> SHMVVLGGDRDFWLQVGIDPIQIMTGTATFYTLRCYLDDRPIFLGRNGRIS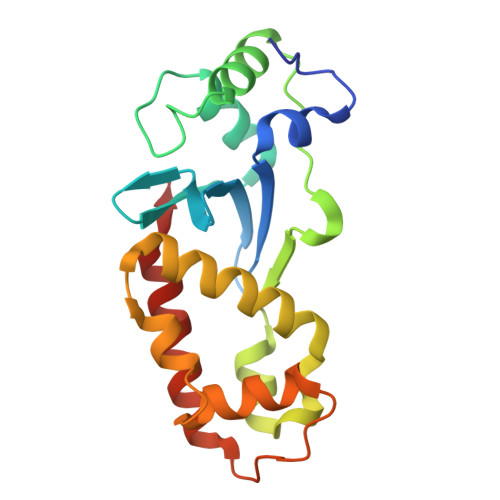VFGSERALARYLADEHDHDLSDLSTYDDIRTAATDGSLAVAVTDDNVYVLSGLVDDFADGPDAVDREQLDLAVELLRDIGDYSEDSAVDKALETTRPLGQLVAYVLDPHSVGKPTAPYAAAVREWEKLERFVESRLRRE>GSHMSSQEIKKIIKRDYSTAPFVLEKITNAIANAMAALGHGSEQDAKLISMQVYESLLNNKEQESEYIPTVEQVQDMVEDKLMSSEFHDVAKAYIIYRNKRALERKTNIFEKRINLKPYEYPELNEYVAAIRHSYWIHTEFNFTSDIQDFKTGLSEVERSAIKNTMLAISQIEVAVKTFWGDVHHRLPKPEIAAVGATFAESEVRHHDAYSHLLEILGLNEEFKELKKKPVIMKRVHYLETSLKHAKSDDDREYTESILLFALFIEHVSLFSQFLIIMAFNKHKNMLKGISNAVEATSKEEQIHGDFGVDIINIIKKENPEWFDEEHNNLIKEMCLNSFEAESKVVDWIFEKG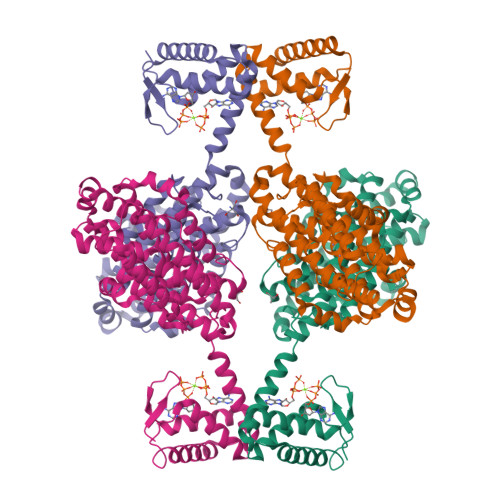ELDFLPKAVINEFLKNRFNKSLEAIGLEKLFDIDEALLQETEWFDDEIIGTKHGDFFVKRSINYSKRTQSITSDDLF[4x]> MASWSHPQFEKGAETAVPNSSSVPGDPSSMRKKNVLLIVVDQWRADFVPHVLRADGKIDFLKTPNLDRLCREGVT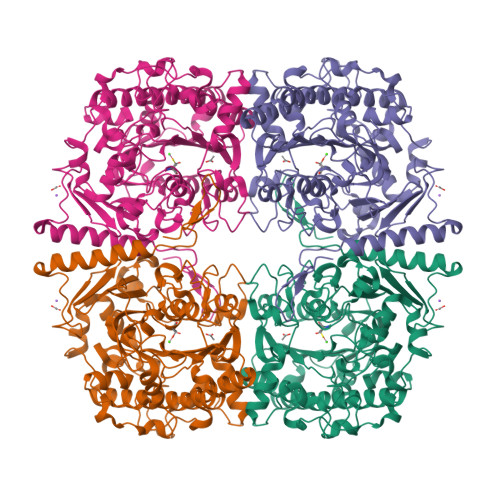FRNHVTTCVPAGPARASLLTGLYLMNHRAVQNTVPLDQRHLNLGKALRGVGYDPALIGYTTTVPDPRTTSPNDPRFRVLGDLMDGFHPVGAFEPNMEGYFGWVAQNGFDLPEHRPDIWLPEGEDAVAGATDRPSRIPKEFSDSTFFTERALTYLKGRDGKPFFLHLGYYRPHPPFVASAPYHAMYRPEDMPAPIRAANPDIEAAQHPLMKFYVDSIRRGSFFQGAEGSGATLDEAELRQMRATYCGLITEVDDCLGRVFSYLDETGQWDDTLIIFTSDHGEQLGDHHLLGKIGYNDPSFRIPLVIKDAGENARAGAIESGFTESIDVMPTILDWLGGKIPHACDGLSLLPFLSEGRPQDWRTELHYEYDFRDVYYSEPQSFLGLGMNDCSLCVIQDERYKYVHFAALPPLFFDLRHDPNEFTNLADDPAYAALVRDYAQKALSWRLKHADRTLTHYRSGPEGLSERSH> AKKKSKLEIIQAILEACKSG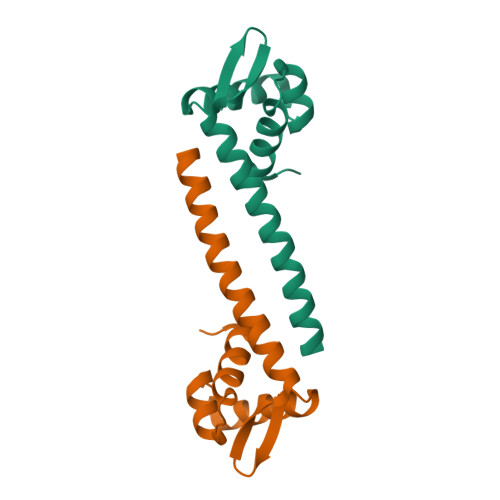SPKTRIMYGANLSYALTGRYIKMLMDLEIIRQEGKQYMLTKKGEELLEDIRKFNEMRKNMDQLKEKINSVLSIRQ>MKVIVVGCTHAGTFAVKQTIADHPDADVTAYEMNDNISFLSCGIALYLGKEIKNNDPRGLFYSSPEELSNLGANVQMRHQVTNVDPETKTIKVKDLITNEEKTEAYDKLIMTTGSKPTVPPIPGIDSSRVYLCKNYNDAKKLFEEAPKAKTITIIGSGYIGAELAEAYSNQNYNVNLIDGHERVLYKYFDKEFTDILAKDYEAHGVNLVLGSKVAAFEEVDDEIITKTLDGKEIKSDIAILCIGFRPNTELLKGKVAMLDNGAIITDEYMHSSNRDIFAAGDSAAVHYNPTNSNAYIPLATNAVRQGRLVGLNLTEDKVKDMGTQSSSGLKLYGRTYVSTGINTALAKANNLKVSEVIIADNYRPEFMLSTDEVLMSLVYDPKTRVILGGALSSMHDVSQSANVLSVCIQNKNTIDDLAMVDMLFQ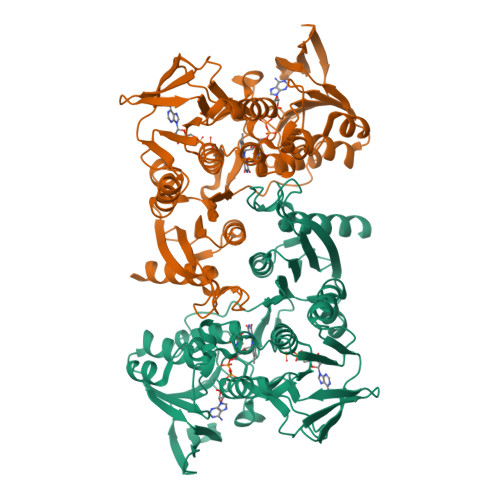PQFDRPFNYLNILGQAAQAQADKAHK[2x]> SMIDDDGYRPNVGIVICNRQGQVMWARRFGQHSWQFPQGGINPGESAEQAMYRELFEEVGLSRKDVRILASTRNW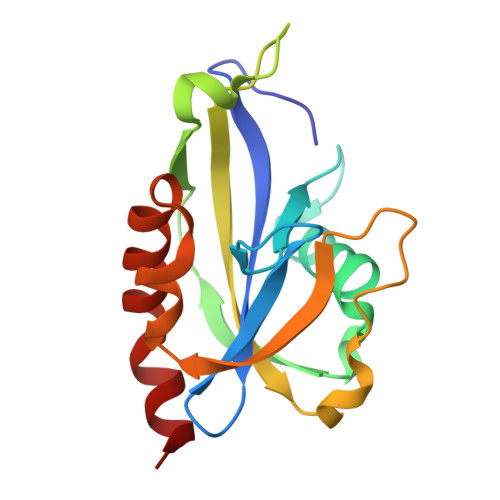LRYKLPKRLVRWDTKPVCIGQKQKWFLLQLVSGDAEINMQTSSTPEFDGWRWVSYWYPVRQVVSFKRDVYRRVMKEFASVVMSLAA> MTSLIDLGRYVERTHHGEDTEPRSKRVKIAKPDLSSFQPGSIIKIRLQDFVTYTLTEFNLSPSLNMIIGPNGSGKSTFVCAVCLGLAGKPEYIGRSKKVEDFIKNGQDVSKIEITLKNSPNVTDIEYIDARDETIKITRIITRSKRRSDYLINDYQVSESVVKTLVAQLNIQLDNLCQFLSQERVEEFARLKSVKLLVETIRSIDASLLDVLDELRELQGNEQSLQKDLDFKKAKIVHLRQESDKLRKSVESLRDFQNKKGEIELHSQLLPYVKVKDHKEKLNIYKEEYERAKANLRAILKDKKPFANTKKTLENQVEELTEKCSLKTDEFLKAKEKINEIFEKLNTIRDEVIKKKNQNEYYRGRTKKLQATIISTKEDFLRSQEILAQTHLPEKSVFEDIDIKRKEIINKEGEIRDLISEIDAKANAINHEMRSIQRQAESKTKSLTTTDKIGILNQDQDLKEVRDAVLMVREHPEMKDKILEPPIMTVSAINAQFAAYLAQCVDYNTSKALTVVDSDSYKLFANPILDKFKVNLRELSSADTTPPVPAETVRDLGFEGYLSDFITGDKRVMKMLCQTSKIHTIPVSRRELTPAQIKKLITPRPNGKILFKRIIHGNRLVDIKQSAYGSKQVFPTDVSIKQTNFYQGSIMSNEQKIRIENEIINLKNEYNDRKSTLDALSNQKSGYRHELSELASKNDDINREAHQLNEIRKKYTMRKSTIETLREKLDQLKREARKDVSQKIKDIDDQIQQLLLKQRHLLSKMASSMKSLKNCQKELISTQILQFEAQNMDVSMNDVIGFFNEREADLKSQYEDKKKFVKEMRDTPEFQSWMREIRSYDQDTKEKLNKVAEKYEEEGNFNLSFVQDVLDKLESEIAMVNHDESAVTILDQVTAELRELEHTVPQQSKDLETIKAKLKEDHAVLEPKLDDIVSKISARFARLFNNVGSAGAVRLEKPKDYAEWKIEIMVKFRDNAPLKKLDSHTQSGGERAVSTVLYMIALQEFTSAPFRVVDEINQGMDSRNERIVHKAMVENACAENTSQYFLITPKLLTGLHYHEKMRIHCVMAGSWIPNPSEDPKMIHFGETSNYSFD;> MISTTISGKRPIEQVDDELLSLTAQQENEEQQQQRKRRRHQFAPMTQFNSNTLDEDSGFRSSSDVATADQDNFLEESPSGYIKKVILRNFMCHEHFELELGSRLNFIVGNNGSGKSAILTAITIGLGAKASETNRGSSLKDLIREGCYSAKIILHLDNSKYGAYQQGIFGNEIIVERIIKRDGPASFSLRSENGKEISNKKKDIQTVVDYFSVPVSNPMCFLSQDAARSFLTASTSQDKYSHFMKGTLLQEITENLLYASAIHDSAQENMALHLENLKSLKAEYEDAKKLLRELNQTSDLNERKMLLQAKSLWIDVAHNTDACKNLENEISGIQQKVDEVTEKIRNRQEKIERYTSDGTTIEAQIDAKVIYVNEKDSEHQNARELLRDVKSRFEKEKSNQAEAQSNIDQGRKKVDALNKTIAHLEEELTKEMGGDKDQMRQELEQLEKANEKLREVNNSLVVSLQDVKNEERDIQHERESELRTISRSIQNKKVELQNIAKGNDTFLMNFDRNMDRLLRTIEQRKNEFETPAIGPLGSLVTIRKGFEKWTRSIQRAISSSLNAFVVSNPKDNRLFRDIMRSCGIRSNIPIVTYCLSQFDYSKGRAHGNYPTIVDALEFSKPEIECLFVDLSRIERIVLIEDKNEARNFLQRNPVNVNMALSLRDRRSGFQLSGGYRLDTVTYQDKIRLKVNSSSDNGTQYLKDLIEQETKELQNIRDRYEEKLSEVRSRLKEIDGRLKSTKNEMRKTNFRMTELKMNVGKVVDTGILNSKINERKNQEQAIASYEAAKEELGLKIEQIAQEAQPIKEQYDSTKLALVEAQDELQQLKEDINSRQSKIQKYKDDTIYYEDKKKVYLENIKKIEVNVAALKEGIQRQIQNACAFCSKERIENVDLPDTQEEIKRELDKVSRMIQKAEKSLGLSQEEVIALFEKCRNKYKEGQKKYMEIDEALNRLHNSLKARDQNYKNAEKGTCFDADMDFRASLKVRKFSGNLSFIKDTKSLEIYILTTNDEKARNVDTLSGGEKSFSQMALLLATWKPMRSRIIALDEFDVFMDQVNRKIGTTLIVKKLKDIARTQTIIITPQDIGKIADIDSSGVSIHRMRDPERQNNSNFYN;> MALNDNPIPKSVPLHPKSGKYFHNLHARDLSNIYQQCYKQIDETINQLVDSTSPSTIGIEEQVADITSTYKLLSTYESESNSFDEHIKDLKKNFKQSSDACPQIDLSTWDKYRTGELTAPKLSELYLNMPTPEPATMVNNTDTLKILKVLPYIWNDPTCVIPDLQNPADEDDLQIEGGKIELTCPITCKPYEAPLISRKCNHVFDRDGIQNYLQGYTTRDCPQAACSQVVSMRDFVRDPIMELRCKIAKMKESQEQDKRSSQAIDVL;> MEVHEEQVSAPVTGDATAKYLLQYILSARGICHENALILALMRLETDASTLNTEWSIQQWVDKLNDYINAINVKLNLLGYKIIRINHGIGRNAVTLKAKQNFESFEDNTAIRAHNNDYAVLQSIVLPESNRFFVYVNLASTEETKLATRFNQNEIEFMKWAIEQFMISGETIVEGPALETSIIVKEVNRILVAATGDSNLAKWRKFSTFTVGSTNLFQFQELTATDIEDLLLRLCELKWFYRTQEGKFGIDLRCIAELEEYLTSMYNLNTCQNCHKLAIQGVR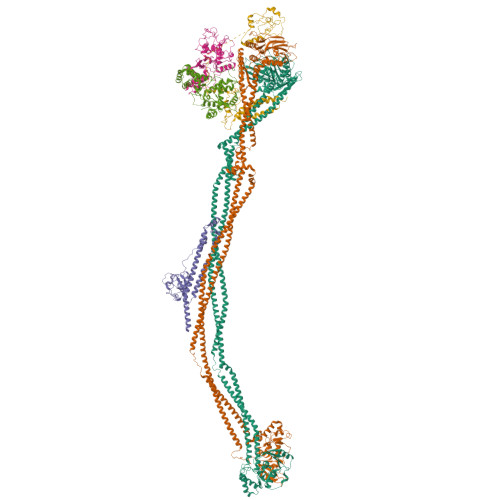CGNESCREENEETGENSLSQIWHVDCFKHYITHVSKNCDRCGSSLITEGVYVI;> MSSIDNDSDVDLTEDLAVAKIVKENPVARKMVRYILSRGESQNSIITRNKLQSVIHEAAREENIAKPSFSKMFMDINAILYNVYGFELQGLPSKNNMNAGGNGSNSNTNKSMPEPLGHRAQKFILLNNVPHSKNFDDFKILQSAHTYEELIVTGEYIGDDIASGTSNTLESKLSTDRDLVYKGVLSVILCIVFFSKNNILHQELIKFLETFGIPSDGSKIAILNITIEDLIKSLEKREYIVRLEEKSDTDGEVISYRIGRRTQAELGLESLEKLVQEIMGLEKEQTKSLHDDIIKSIGDSYSI;> MSSTVISRKRRNSTVTEPDSSGETRKQKKSRSDEKSSSSKDGDPQLEFKVLQGYRDLESEMHKGRAQVTRTGDIGVAMDNLNAVDSLFNKVIGIKNNGLFAHDARAMVSISELAQISVRNLKFDDSRSMVNLENIVNSLKRYMLKEHFKLNNIAENRNDLTLAADEQSAADQQEESDGDIDRTPDDNHTDKATSSFKATSMRHSYLQQFSHYNEFSQFNWFRIGALYNTISKNAPITDHLMGPLSIEKKPRVLTQRRRNNDQVGEKITAEKITQHSLNSTQQETTPEQVKKCFKKLSKKLGPEGSINLFKFIIDPNSFSRSIENLFYTSFLIKEGKLLMEHDEEGLPTIKIKQSISHTDSRSKEIERQRRRAAHQNHIIFQMDMPTWRKLIKKYNITSPFLD The hyperthermophilic endocellulase, EGPh (glycosyl hydrolase family 5) from Pyrococcus horikoshii possesses 4 cysteine residues forming 2 disulfide bonds, as identified by structural analysis. The crystal structure of hyperthermophilic beta-1,4 endocellulases (EGPh, glycosyl hydrolase family 5, T opt = 100 °C) from the archaeon Pyrococcus horikoshii, that was isolated from an oceanic hydrothermal volcanic vent, has been determined. The crystal structure of EGPh revealed 4 Cys residues (C106, C159, C372, and C412) forming 2 disulfide bonds. The disulfide bonding of C106 and C159 forms at the end of the loop associated with the substrate-binding active site cleft.

To investigate a role of the disulfide bond in the activity and stability of the enzyme, we prepared 3 mutants of EGPh; P74C, C106S, and P74C/C106S, in which we removed the disulfide bond or changed the disulfide-bonding pattern. The mutant P74C/C106S possesses 2 Cys residues at the region and is expected to form a disulfide bond (C74–C159) structurally similar to that of EGAc (C34–C120). Moreover, as expected, the P74C/C106S mutation possesses an identical disulfide bond (C74–C159) conserved in EGAc. The crystal structural analysis of EGPh mutants revealed that a new disulfide bond at the position of P74 is formed in P74C and P74C/C106S. No significant change in the enzymatic activity at 80 °C was observed between the mutants and the wild type (data not shown), suggesting that the region involving the disulfide bond did not significantly influence substrate-binding or catalysis. All of the mutants showed a dramatic decrease in residual activity after heat treatment compared with the wild type. The wild type enzyme was thermally unfolded at 103.4 °C. The melting temperature of the 3 mutants was approximately 101.5 °C. These results indicate that the alternative new disulfide-bonding pattern involved in the position of P74 did not contribute to its hyperthermostability. However, the thermal analysis indicates that the C106–C159 bond with higher potential energy contributes to thermostability while the C74–C159 bond has no role in stability.

>[3x]QTPTGIYYEVRGDTIYMINVTSGEETPIHLFGVNWFGFETCNHVVHGLWKRNWEDMLLQIKSLGFNAIRLPFCTESVKPGTQPIGIDYSKNPDLRGLDSLQIMEKIIKKAGDLGIFVLLDYHRIGCTHIEPLWYTEDFSEEDFINTWIEVAKRFGKYWNVIGADLKNEPHSVTSPPAAYTDGTGATWGMGNPATDWNLAAERIGKAILKVAPHWLIFVEGTQFTNPKTDSSYKWGYNAWWGGNLMAVKDYPVNLPKNKLVYSPHVYGPDVYNQPYFGPAKGFPDNLPDIWYHHFGYVKLELGYSVVIGEFGGKYGHGGDPRDVIWQNKLVDWMIENKFCDFFYWSWNPDSGDTGGILQDDWTTIWEDKYNNLKRLMD> MHHHHHHVMIMKAFISENVRGIYAFDENGNLIEKRYFTDKPEKVLDQLLKGEITKDLEELLNSLKEKGYDEFVFEHPELSRRAKELGFSATTEFPNIAGERLRSNPEEFLGENWFEEYYKVGVALTRMRIQEQSGARDKMVIQAIEALDDVDKVINLL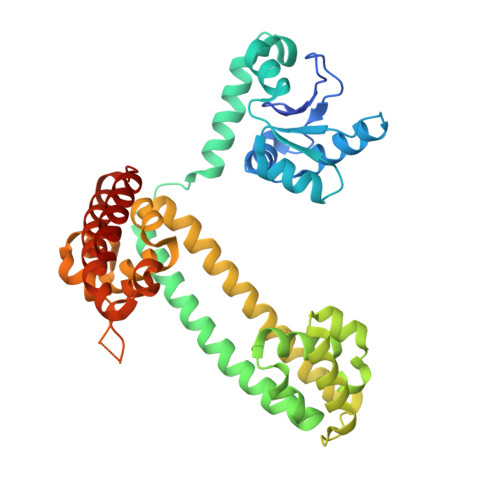VARLREWYSLHFPELDELLPKHPQYVAFVKTVGHRDNINEEVLRELGLSEEKIKKILEAKEKTMGAWMDQTDIEVVRQLAEEIDRLYQLRKKLEDYIDRAMDDVAPNLKALVGAKLAARLISLAGGLRELAMMPSSTIQVLGAEKALFRHLRTGAKPPKHGVIYQYPAINRSPWWQRGKIARALAGKLAIAARVDYFSGEYIAEELKKELEARIREIK>MLEGLSWVDYGERAELDDSDGHGNHRESSPFLSPLEASRGIDYYDRNLALFEEELDIRPKVSSLLGKLVSYTNLTQGAKEHEEAESGEGTRRRAAEAPSMGTLMGVYLPCLQNIFGVILFLRLTWMVGTAGVLQALLIVLICCCCTLLTAISMSAIATNGVVPAGGSYFMISRSLGPEFGGAVGLCFYLGTTFAAAMYILGAIEILLTYIAPPAAIFYPSGAHDTSNATLNNMRVYGTIFLTFMTLVVFVGVKYVNKFASLFLACVIISILSIYAGGIKSIFDPPVFPVCMLGNRTLSRDQFDICAKTAVVDNETVATQLWSFFCHSPNLTTDSCDPYFMLNNVTEIPGIPGAAAGVLQENLWSAYLEKGDIVEKHGLPSADAPSLKESLPLYVVADIATSFTVLVGIFFPSVTGIMAGSNRSGDLRDAQKSIPVGTILAIITTSLVYFSSVVLFGACIEGVVLRDKYGDGVSRNLVVGTLAWPSPWVIVIGSFFSTCGAGLQSLTGAPRLLQAIAKDNIIPFLRVFGHGKVNGEPTWALLLTALIAELGILIASLDMVAPILSMFFLMCYLFVNLACAVQTLLRTPNWRPRFKYYHWALSFLGMSLCLALMFVSSWYYALVAMLIAGMIYKYIEYQGAEKEWGDGIRGLSLSAARYALLRLEEGPPHTKNWRPQLLVLLKLDEDLHVKYPRLLTFASQLKAGKGLTIVGSVIQGSFLESYGEAQAAEQTIKNMMEIEKVKGFCQVVVASKVREGLAHLIQSCGLGGMRHNSVVLGWPYGWRQSEDPRAWKTFIDTVRCTTAAHLALLVPKNIAFYPSNHERYLEGHIDVWWIVHDGGMLMLLPFLLRQHKVWRKCRMRIFTVAQMDDNSIQMKKDLAVFLYHLRLEAEVEVVEMHNSDISAYTYERTLMMEQRSQMLRQMRLTKTEREREAQLVKDRHSALRLESLYSDEEDESAVGADKIQMTWTRDKYMTETWDPSHAPDNFRELVHIKPDQSNVRRMHTAVKLNEVIVTRSHDARLVLLNMPGPP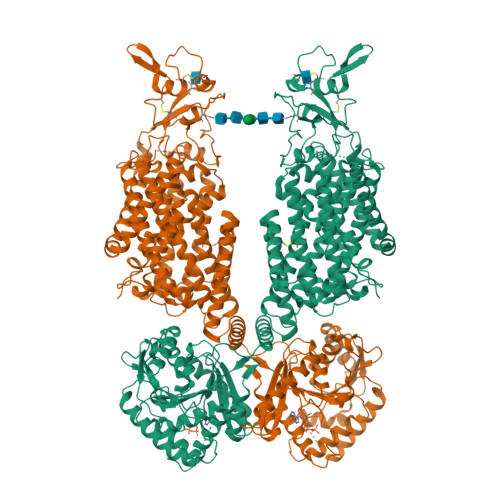RNSEGDENYMEFLEVLTEGLERVLLVRGGGREVITIYSAENLYFQ[2x]> NLYQFKNMIKCTVPSRSWWDFADYGCYCGRGGSGTPVDDLDRCCQVHDNCYNEAEKISGCWPYFKTYSYECSQGTLTCKGDNNACAASVCDCDRLAAICFAGAPYNDNNYNID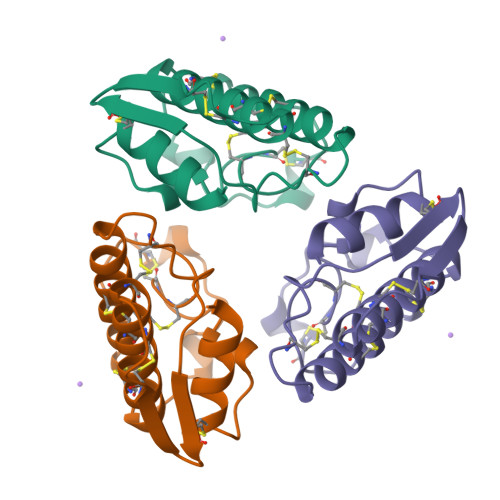LKARCQ>[2x]SNAMHNVVITAAVRSPIGTFGGALKNVTPVELAVPVLQEAVKRGGVEPHEVDEVILGHCIQRTDEANTARTAALAAGFPDTVTGYTIQRQCSSGMQAIMSAAMQIQLGVSEVVVAGGVEAMSSSPYALKQHRWGQRLQHGEIRDTVWEVLEDPIHHIMMGETAENLVEQYEITREEQDEVALRSHTLALKAIESGYFDDQIVPITIKERR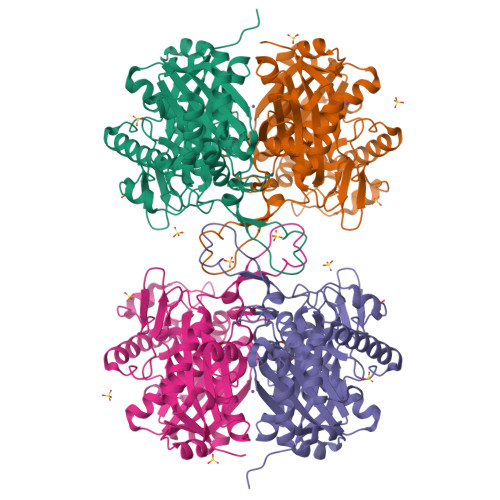KEVVFSKDEHPRADITAEKLAGLKPAFRKDGSVTAGNASGLNDGSAVLVLMSEEKAKEKGLQPLARIVGYSVAGVDPKIMGIGPAPAIRKGLEKVDWSLEDADLLEINEAFAAQYLAVEKELDLDREKVNVNGSGVGLGHPIGCTGARITVSLIHELKRRGLEKGIASLCVGGGIGVALFIEAL Mycobacterium tuberculosis (MTB) H37Rv is predicted to encode three COMTs, i.e., Rv1220, Rv1703, and Rv0187, which share 29 to 36% amino acid sequence identity. Here, we present two crystal structures of Rv0187 from MTB H37Rv with and without cofactors at 1.64 and 2.08 Å resolution, respectively. The protein adopts the Rossmann fold typical for numerous SAM-dependent methyltransferases, containing seven core β-sheets surrounded by eight α-helices (α1α2α3β1α4β2α5β3α6β4α7β5α8β6β7). In both ligand-free and cofactor-bound structures, Rv0187 appears to form a canonical dimer observed for all known COMT structures, consistent with the results of our SEC experiments.

Meanwhile, the ASU of the cofactor-bound structure is composed of eight monomers, and each subunit exhibits the unambiguous presence of a divalent metal ion and SAH. At the initial stage of model building from X-ray diffraction data, excessive electron density around the modeled magnesium ion was observed in the Fo-Fc difference Fourier map, signifying the presence of a more electron-rich element despite magnesium salt being added to the protein sample. Since strontium chloride was included in the crystallization cocktail solution, the extra electron density most likely arose from Sr2+. Therefore, Sr2+ was included in the model for the subsequent refinement stages in place of Mg2+. Pseudobipyramidal geometry of strontium coordination is observed, similar to the octahedral coordination of magnesium or calcium in other COMT structures. In the cofactor-bound structure of Rv0187, a strontium ion is complexed by Asp-139, Asp-165, Asn-166, two water molecules, and Asp-178 of an adjacent subunit, which is non-crystallographically related. Located close to the metal binding site is SAH, a product from COMT-dependent methyltransfer reactions, where the sulfur atom is approximately 5.3 Å distant from the Sr2+. The overall binding pose of SAH is essentially identical, with slight variations in each subunit. The hydrogen-bonding interaction between the N1 of the adenine moiety and the backbone amide group of Ala-121 is universally conserved in all eight chains. The amine group of the methionyl moiety forms hydrogen bonds with the backbone carbonyl oxygen of Gly-68 and with the side chains of Asp-139 and Ser-74.

>[8x]MGMDQQPNPPDVDAFLDSTLVGDDPALAAALAASDAAELPRIAVSAQQGKFLCLLAGAIQARRVLEIGTLGGFSTIWLARGAGPQGRVVTLEYQPKHAEVARVNLQRAGVADRVEVVVGPALDTLPTLAGGPFDLVFIDADKENNVAYIQWAIRLARRGAVIVVDNVIRGGGILAESDDADAVAARRTLQMMGEHPGLDATAIQTVGRKGWDGFALALVRENLYFQGGHHHHHHG>SNAMKADILLVSHSKMITDGIKEMIEQMNASEEITIHSLGGTSDGSLG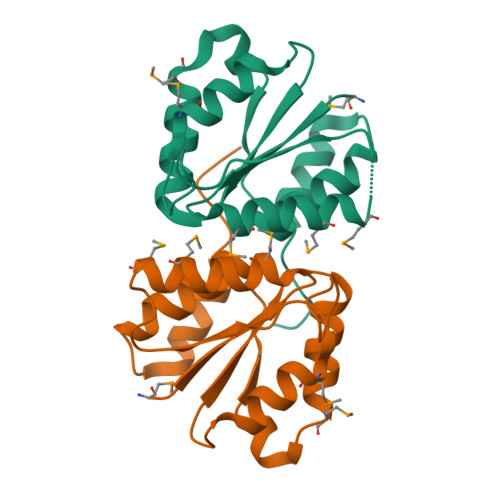SDPMKIIDTINEADSDREFLIFADLGSAVLSSELAFDMLEEDQQKHYHLVDAPLVEGAFASAITAGVSDDLTQILAEAQNAGKKGWN[6x]> MGDCDIEGKDGKQYESVLMVSIDQLLDSMKEIGSNCL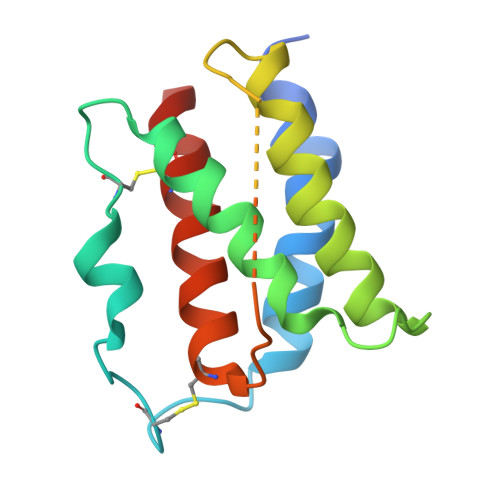NNEFNFFKRHICDANKEGMFLFRAARKLRQFLKMNSTGDFDLHLLKVSEGTTILLNCTGQVKGRKPAALGAAQPTKSLEENKSLKEQKKLNDLCFLKRLLQEIKTCWNKILMGTKEH> MAFHWCDNNLHTTVFTPRDFQVELLATAYERNTIICLGHRSSKEFIALKLLQELSRRARRHGRVSVYLSCEVGTSTEPCSIYTMLTHLTDLRVWQEQPDMQIPFDHCWTDYHVSILRPEGFLYLLETRELLLSRVELIVLEDCHDSAVYQRIRPLFENHIMPAPPADRPRILGLAGPLHSAGCELQQLSAMLATLEQSVLCQIESASDIVTVLRYCSRPHEYIVQCAPFEMDELSLVLADVLNTHKSFLLDHRYDPYEIYGTDQFMDELKDIPDPKVDPLNVINSLLVVLHEMGPWCTQRAAHHFYQCNEKLKVKTPHERHYLLYCLVSTALIQLYSLCEHAFHRHLGSGSDSRQTIERYSSPKVRRLLQTLRCFKPEEVHTQADGLRRMRHQVDQADFNRLSHTLESKCRMVDQLDQPPTETRALVATLEQILHTTEDRQTNRSAARVTPTPTPAHAKPKPSSGANTAQPRTRRRVYTRRHHRDHNDGSDTLCALIYCNQNHTARVLFELLAEISRRDPDLKFLRCQYTTDRVADPTTEPKEAELEHRRQEEVLKRFRMHDCNVLIGTSVLEEGIDVPKCNLVVRWDPPTTYRSYVQCKGRARAAPAYHVILVAPSYKSPTVGSVQLTDRSHRYICATGDTTEADSDSDDSAMPNSSGSDPYTFGTARGTVKILNPEVFSKQPPTACDIKLQEIQDELPASAQLDTSNSSDEAVSMSNTSPSESSTEQKSRRFQCELSSLTEPEDTSDTTAEIDTAHSLASTTKDLVHQMAQYREIEQMLLSKCANTEPPEQEQCEAERFSACLAAYRPKPHLLTGASVDLGSAIALVNKYCARLPSDTFTKLTALWRCTRNERAGVTLFQYTLRLPINSPLKHDIVGLPMPTQTLARRLAALQACVELHRIGELDDQLQPIGKEGFRALEPDWECFELEPEDEQIVQLSDEPRPGTTKRRQYYYKRIASEFCDCRPVAGAPCYLYFIQLTLQCPIPEEQNTRGRKIYPPEDAQQGFGILTTKRIPKLSAFSIFTRSGEVKVSLELAKERVILTSEQIVCINGFLNYTFTNVLRLQKFLMLFDPDSTENCVFIVPTVKAPAGGKHIDWQFLELIQANGNTMPRAVPDEERQAQPFDPQRFQDAVVMPWYRNQDQPQYFYVAEICPHLSPLSCFPGDNYRTFKHYYLVKYGLTIQNTSQPLLDVDHTSARLNFLTPRYVNRKGVALPTSSEETKRAKRENLEQKQILVPELCTVHPFPASLWRTAVCLPCILYRINGLLLADDIRKQVSADLGLGRQQIEDEDFEWPMLDFGWSLSEVLKKSRESKQKESLKDDTINGKDLVDVEKKAISEETQIDKDSKDDKVEKSAIELIIEGEEKLQEADDFIEIGTWSNDMADDIASFNQEDDDEDDAFHLPVLPANVKFCDQQTRYGSPTFWDVSNGESGFKGPKSSQNKQGGKGKAKGPAKPTFNYYDSDNSLGSSYDDDDNAGPLNYMHHNYSSDDDDVADDIDAGRIAFTSKNEAETIETAQEVEKRQKQLSIIQATNANERQYQQTKNLLIGFNFKHEDQKEPATIRYEESIAKLKTEIESGGMLVPHDQQLVLKRSDAAEAQVAKVSMMELLKQLLPYVNEDVLAKKLGDRRELLLSDLVELNADWVARHEQETYNVMGCGDSFDNYNDHHRLNLDEKQLKLQYERIEIEPPTSTKAITSAILPAGFSFDRQPDLVGHPGPSPSIILQALTMSNANDGINLERLETIGDSFLKYAITTYLYITYENVHEGKLSHLRSKQVANLNLYRLGRRKRLGEYMIATKFEPHDNWLPPCYYVPKELEKALIEAKIPTHHWKLADLLDIKNLSSVQICEMVREKADALGLEQNGGAQNGQLDDSNDSCNDFSCFIPYNLVSQHSIPDKSIADCVEALIGAYLIECGPRGALLFMAWLGVRVLPITRQLDGGNQEQRIPGSTKPNAENVVTVYGAWPTPRSPLLHFAPNATEELDQLLSGFEEFEESLGYKFRDRSYLLQAMTHASYTPNRLTDCYQRLEFLGDAVLDYLITRHLYEDPRQHSPGALTDLRSALVNNTIFASLAVRHGFHKFFRHLSPG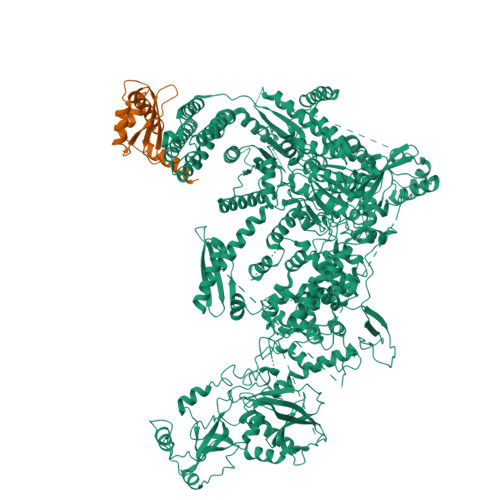LNDVIDRFVRIQQENGHCISEEYYLLSEEECDDAEDVEVPKALGDVFESIAGAIFLDSNMSLDVVWHVYSNMMSPEIEQFSNSVPKSPIRELLELEPETAKFGKPEKLADGRRVRVTVDVFCKGTFRGIGRNYRIAKCTAAKCALRQLKKQGLIAKKD;> MDQENFHGSSLPQQLQNLHIQPQQASPNPVQTGFAPRRHYNNLVGLGNGNAVSGSPVKGAPLGQRHVKLKKEKISAQVAQLSQPGQLQLSDVGDPALAGGSGLQGGVGLMGVILPSDEALKFVSETDANGLAMKTPVSILQELLSRRGITPGYELVQIEGAIHEPTFRFRVSFKDKDTPFTAMGAGRSKKEAKHAAARALIDKLIGAQLPESPSSSAGPSVTGLTVAGSGGDGNANATGGGDASDKTVGNPIGWLQEMCMQRRWPPPSYETETEVGLPHERLFTIACSILNYREMGKGKSKKIAKRLAAHRMWMRLQETPIDSGKISDSICGELEGEPRSSENYYGELKDISVPTLTTQHSNKVSQFHKTLKNATGKKLLKLQKTCLKNNKIDYIKLLGEIATENQFEVTYVDIEEKTFSGQFQCLVQLSTLPVGVCHGSGPTAADAQRHAAQNALEYLKIMTKK Dihydroxy acid dehydratase (DHAD) is the third enzyme in the plant branched-chain amino acid biosynthetic pathway and the target for commercial herbicide development. We have previously reported the discovery of fungal natural product aspterric acid (AA) as a submicromolar inhibitor of DHAD through self-resistance gene directed genome mining. Here, we reveal the mechanism of AA inhibition on DHAD and the self-resistance mechanism of AstD, which is encoded by the self-resistance gene astD. Our structural and kinetic analysis of the mutant AthDHADs has validated the hypothesis that larger hydrophobic amino acids surrounding the active-site entrance enhance resistance to AA.

To determine if small-to-large amino acid mutations at these hydrophobic residues can decrease active site volume and increase resistance to AA, we generated multiple mutations at V496, V497, and I177 in AthDHAD followed by kinetic and structural characterizations. The substitution of I177L might result in smaller active cavity. TI177L and I177F mutants had an IC50 of 0.05 and 37.0 μM. To probe the acquired resistance mechanism of AthDHAD mutants, we determined the crystal of AthDHAD–I177F (2.45 Å), AthDHAD–V178W (1.77 Å), AthDHAD–V496W (1.59 Å), and AthDHAD–V497F (1.87 Å). In the crystal structures of I177F, V178W, V496W, and V497F, the occupancy of [2Fe–2S] cluster is 0.64, 0.72, 0.63, and 0.77, respectively. The overall structures of the AthDHAD mutants I177F, V178W, V496W, and V497F displayed high similarity with the wild-type AthDHAD, with the RMSD of 0.123 Å (888 core Cα atoms), 0.275 Å (994 core Cα atoms), 0.142 Å (1,034 core Cα atoms), and 0.283 Å (994 core Cα atoms), respectively. As a result, this mutant also affects the accession of AA to the active site. Both V178 and I177 are close to the active site. I177F make the cavity smaller, so that the cavity cannot accommodate the hydrophobic part of AA.

> GSIISCSAQSVTADPSPPITDTNKLNKYSSRITEPKSQGGSQAILHGVGLSDDDLLKPQIGISSVWYEGNTCNMHLLKLSEAVKEGVENAGMVGFRFNTIGVSDAISMGTRGMCFSLQSRDLIADSIETVMSAQWYDGNISIPGCDKNMPGTIMAMGRLNRPGIMVYGGTIKPGHFQDKTYDFVSAFQSYGEFVSGSISDEQRKTVLHHSCPGAGACGGMYTANTMASAIEAMGMSLPYSSSIPAEDPLKLDECRLAGKYLLELLKMDLKPRDIITPKSLRNAMVSVMALGGSTNAVLHLIAIARSVGLELTLDDFQKVSDAVPFLADLKPSGKYVMEDIHKIGGTPAVLRYLLELGLMDGDCMTVTGQTLAQNLENVPSLTEGQEIIRPLSNPIKETGHIQILRGDLAPDGSVAKITGKEGLYFSGPALVFEGEESMLAAISADPMSFKGTVVVIRGEGPKGGPGMPEMLTPTSAIMGAGLGKECALLTDGRFSGGSHGFVVGHICPEAQEGGPIGLIKNGDIITIDIGAARIDTQVSPEEMNDRRKKWTAPAYKVNRGVLYKYIKNVQSASDGCVTDE> DKMPDWNIPSLYE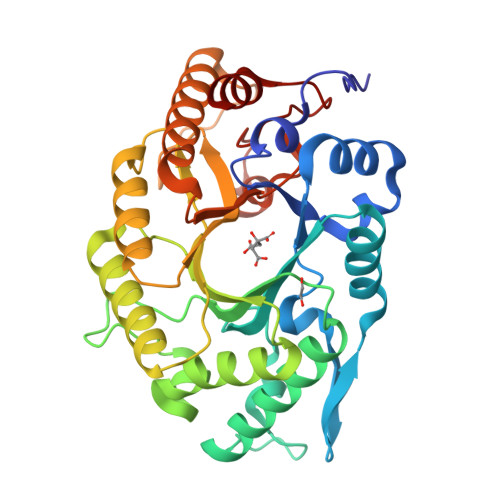SYKNDFRIGVAIPAKCLSNDTDRRMVLKHFNSITAENEMKPESLLAGQTSTGLNYRFSTADTFVDFANTNNIGIRGHTLVWHSQTPDWFFKDSSGQRLTKDALLARLKQYIYDVVGRYKGKVYAWDVVNEAIDENQSDGYRRSTWYEICGPEYIEKAFIWAHEADPNAKLFYNDYNTEISKKRDFIYNMVKNLKSKGIPIHGIGMQCHINVNWPSVSEIENSIKLFSSIPGIEIHITELDMSLYNYGSSENYSTPPQDLLQKQAQKYKELFTMLKKYTNVVKCVTFWGLKDDYSWLRSFNGKNDWPLLLFEDYSAKPAYWAVIEAS> HHHHHHMRVLGLNGWPRDFHDASAALLVDGRIAAFAEEERFTRKKHGYNTAPVQAAAFCLAQAGLTVDDLDAVAFGWDLPAMYRERLGGWPHSDSEALDILLPRDVFPRRTDPPLHFVQHHLAHAASAYYFSGEDRGAVLIVDGQGEEECVTLAHAEGGKITVLDTVPGAWSLGFFYEHVSEYTGLGGDNPGKLMGLAAHGTTVDETLSAFAFDSDGYRLNLIDPQARDPEDWDEYSVTERAWFAHLERIYRLPPNEFVRRYDPAKGRVVRDTRRDPYEYRDLAATAQAALERAVFGLADSVLARTGERTLFVAGGVGLNATMNGKLLTRSTVDKMFVPP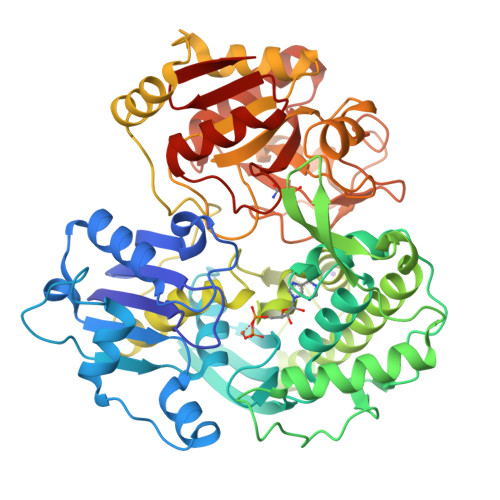VASDIGVSLGAAAAVAVELGDRIAPMGDTAAWGPEFSPDQVRAALDRTGLAYREPANLEREVAALIASGKVVGWAQGRGEVGPRALGQRSLLGSAHSPTMRDHINLRVKDREWWRPFAPSMLRSVSDQVLEVDADFPYMIMTTKVRAAYAERLPSVVHEDWSTRPQTVTEASNPRYHRMLTELGDLVGDPVCLNTAFNDRGEPIVSSPADALLTFSRLPIDALAVGPYLVTKDLRH>[4x]GPGSEIQVLKAPRAVVWKDFLGVNAQFLWFSPERYNKQIDRLQDLGLEWVRLDLHWDRLETAEDQYQLASLDQLVKDLEARQLKSVFYLV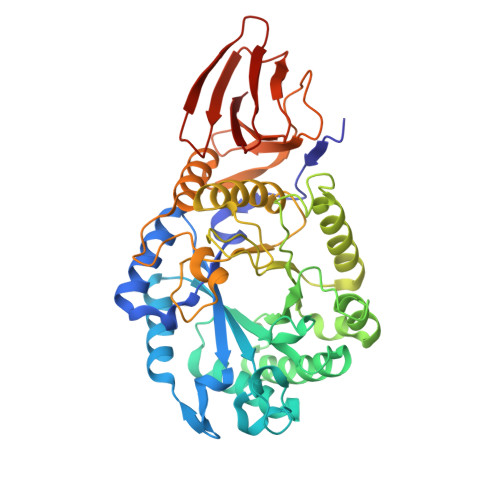GSARFITTAPFYSPFQDQYPPRDPEVFARRMAMLSQRYPSVAAWQVWNEPNLIGFWRPKADPEGYAKLLQASTIALRMVDPEKPVVSAGMAFFSEMPDGRTMFDALGHLGVESLGTIATYHPYTQLPEGNYPWNLDFVSHANQINRALRNAGVPAIWSTEWGWSAYKGPKELQDIIGVEGQADYVLRRLALMSALDYDRIFLFTLSDLDQRASVRDRDYGLLDLDANPKPVYLALQRFLKVTGPKLRPADPPVTEDLPDGSFSIGWTREDGRNVWLFWSARGGNVRLPKLKEATLHDPLSGKVTPLSGSDGLEVPVKSSLQMLVWE> XCHP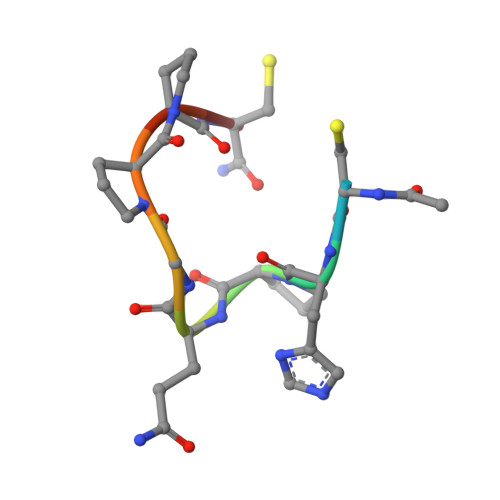QGPPCX>HCALPCGVYDPAQARIEAESVKAVQEKMAGNDDPHFQTRATVIKEQRAELAKHHVSVLWSDYFKP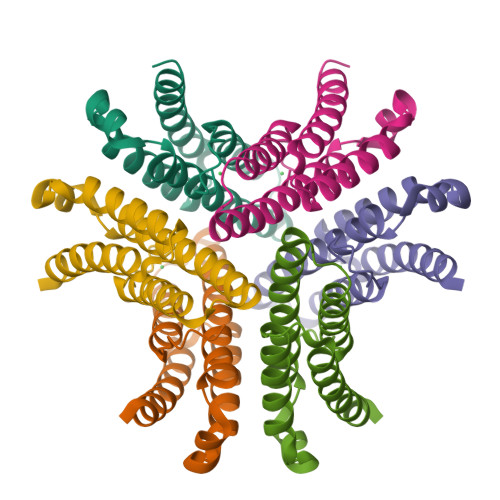PHFEKYPELHQLVNDTLKALSAAKGSKDPATGQKALDYIAQIDKIFWETKKA[3x]>EQTNQIANKPQAIQWHTNLTNERFTTIAHRGASGYAPEHTFQAYDKSHNELKASYIEIDLQRTKDGHLVAMHDETVNRTTNGHGKVEDYTLDELKQLDAG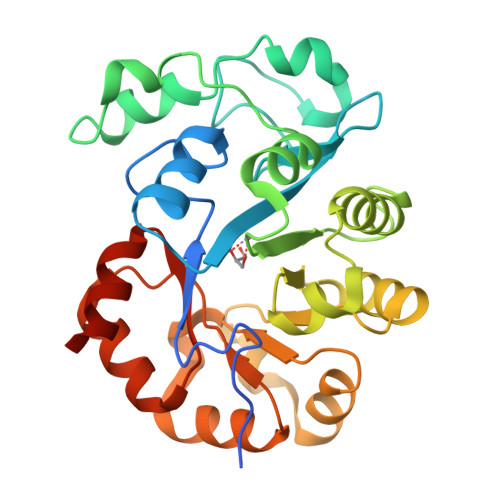SWFNKKYPKYARASYKNAKVPTLDEILERYGPNANYYIETKSPDVYPGMEEQLLASLKKHHLLNNNKLKNGHVMIQSFSDESLKKIHRQNKHVPLVKLVDKGELQQFNDQRLKEIRSYAIGLGPDYTDLTEQNTHHLKDLGFIVHPYTVNEKADMLRLNKYGVDGVFTNFADKYKEVIKEGHHHHHH[8x]> MGSSHHHHHHSSGENLYFQGHESGSKEVT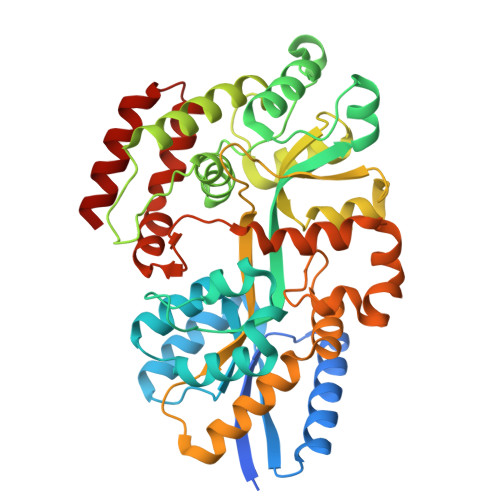IEFMHSSVEKERLDVINKLIADFEKENPTIKIKQIPVEEDAFNTKVVTLARSGKLPAVMEVSQDFAKVMDKDELIDQDAVKEVIDSVGEDKYYEGATNLVRSEDGKSYIAAPLSGWVQGIWYNKKALADAGFEEPKNWADIEKVAKKFTNKADKKYGIAIPTAESTMSEQAFSQFALSNKANVLDAKGNVTIDTPEMKEALQYYKDLSAYTMPGSNDVTEIKDAFMNGTVPMAMYSTYILPSVYEEGDPKNIGFAIPEEKEKAVYGTVSGLTISAGLDDEQKKATKKFVEYLSQPENMATWVLMSPGGAQPVNKEVVEQKAYKENEVIKSFGDLPNEIAASFNDIQVFGLVDGKNLTKMGDITSSGIIAQMVNNVTVGGGDVSADLKAAQKKAEEGK>[4x]MVSAGIEAMNVFGGTAYLDVMELAKYRHLDTARFENLLMKEKAVALPYEDPVTFGVNAAKPIIDALSEAEKDRIELLITCSE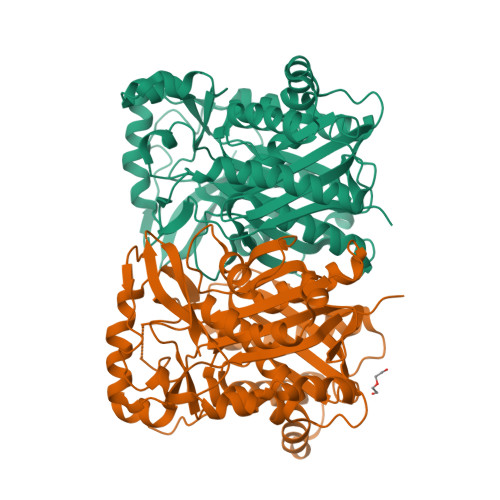SGIDFGKSLSTYIHEYLGLNRNCRLFEVKQACYSGTAGFQMAVNFILSQTSPGAKALVIASDISRFLIAEGGDALSEDWSYAEPSAGAGAVAVLVGENPEVFQIDPGANGYYGYEVMDTCRPIPDSEAGDSDLSLMSYLDCCEQTFLEYQKRVPGANYQDTFQYLAYHTPFGGMVKGAHRTMMRKVAKVKTSGIETDFLTRVKPGLNYCQRVGNIMGAALFLALASTIDQGRFDTPKRIGCFSYGSGCCSEFYSGITTPQGQERQRTFGIEKHLDRRYQLSMEEYELLFKGSGMVRFGTRNVKLDFEMIPGIMQSTQEKPRLFLEEISEFHRKYRWIS>SGGGMLTLIQGKKIVNHLRSRLAFEYNGQLIKILSKNIVAVGSLRREEKMLNDVDLLIIVPEKKLLKHVLPNIRIKGLSFSVKVCGERKCVLFIEWEKKTYQLDLFTALAEEKPYAIFHFTGPVSYLIRIRAALKKKNYKLNQYGLFKNQTLVPLKITTEKEL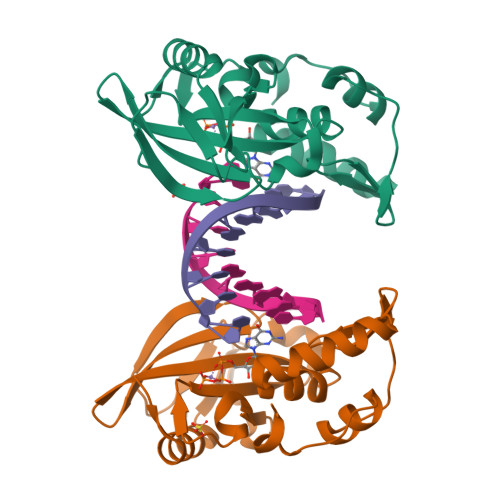IKELGFTYRIPKKRL[2x]In this article we describe the crystal structure of TarS, an enzyme responsible for the glycosylation of wall teichoic acid polymers of the S. aureus cell wall, a process that has been shown to be specifically responsible for methicillin resistance in MRSA. TarS possesses a catalytic domain with a canonical GTA fold (one of two distinct A/B folds characteristic of nucleotide-sugar dependent glycosyltransferases) consisting of two closely associated α/β/α sandwich Rossmann motifs that abut and form a continuous central β-sheet. TarS possesses a D(91)XDD motif with aspartates coordinating a metal cation, a feature that is typical of the GTA superfamily. Altogether, TarS features a novel architecture with closely-associated trimerization domains connected by a linker region to three protruding catalytic domains that face away from each other.

The full-length TarS crystals diffracted with strong anisotropy and a high resolution limit of 4 Å was applied. The higher resolution TarS1-349 and TarS217-573 structures were subsequently used as molecular replacement search models to solve the structure of the full-length TarS, revealing a “hanging basket” like structure with variation in the relative domain orientation of the three catalytic domains with respect to the trimerization domain. Although TarS was co-crystallized in the presence of the UDP-GlcNAc sugar donor, only the cleaved UDP product seemed to be observed (ligand mFo-dFc simulated annealing omit electron density shown in S2C Fig) and the crystals were too sensitive to withstand soaking in higher concentrations of UDP-GlcNAc as for the TarS1-349 crystals. In light of the data quality, refinement was closely monitored using the higher resolution structures as restraints and validated by the visualization of OMIT maps for both protein and ligands. The structure of full-length TarS suggests motion between the catalytic domains and corresponding trimerization domains, where an overlay of trimer monomers reveals varying angles (50° vs. 64° vs. 78° as measured with the UCSF Chimera package) between the common plane of the trimerization domain and the individual planes of the catatlytic domains, with the hinge point centered on P352. The difference in angles is unlikely to have resulted from crystal packing artifacts, given that the catalytic domains in the full-length structure are not involved in any crystal contacts. We propose therefore that the apparent flexibility between the two domains may be related to substrate binding and/or processivity. TarS furthermore displays a pronounced electrostatic sidedness, which may be related to membrane localization or substrate/partner interactions. The physiological relevance of the trimeric architecture is supported by size exclusion chromatography-multiangle light scattering (SECMALS) with an elution profile that corresponds predominantly to a 200 kDa species (theoretical monomer molecular weight is 66 kDa).

>MKFSVIVPTYNSEKYITELLNSLAKQDFPKTEFEVVVVDDCSTDQTLQIVEKYRNKLNLKVSQLETNSGGPGKPRNVALKQAEGEFVLFVDSDDYINKETLKDAAAFIDEHHSDVLLIKMKGVNGRGVPQSMFKETAPEVTLLNSRIIYTLSPTKIYRTALLKDNDIYFPEELKSAEDQLFTMKAYLNANRISVLSDKAYYYATKREGEHMSSAYVSPEDFYEVMRLIAVEILNADLEEAHKDQILAEFLNRHFSFSRTNGFSLKVKLEEQPQWINALGDFIQAVPERVDALVMSKLRPLLHYARAKDIDNYRTVEESYRQGQYYRFDIVDGKLNIQFNEGEPYFEGIDIAKPKVKMTAFKFDNHKIVTELTLNEFMIGEGHYDVRLKLHSRNKKHTMYVPLSVNANKQYRFNIMLEDIKAYLPKEKIWDVFLEVQIGTEVFEVRVGNQRNKYAYTAETSALIHLNNDFYRLTPYFTKDFNNISLYFTAITLTDSISMKLKGKNKIILTGLDRGYVFEEGMASVVLKDDMIMGMLSQTSENEVEILLSKDIKKRDFKNIVKLNTAHMTYSLK[3x]> ASKEEVPDNPPNEIYATAQQKLQDGNWRQAITQLEALDNRYPFGPYSQQVQLDLIYAYYKNADLPLAQAAIDRFIRLNPTHPNIDYVMYMRGLTNMA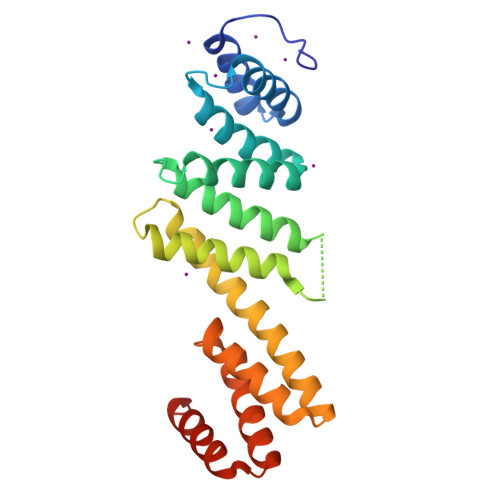LDDSALQGFFGVDRSDRDPQHARAAFSDFSKLVRGYPNSQYTTDATKRLVFLKDRLAKYEYSVAEYYTERGAWVAVVNRVEGMLRDYPDTQATRDALPLMENAYRQMQMNAQAEKVAKIIAANSSNT> GSAGTSTATNAGPLLQRVGGLDVVKKVVELFYRKLYADPQLIKYLHDQDPMHLRAKQSMFVS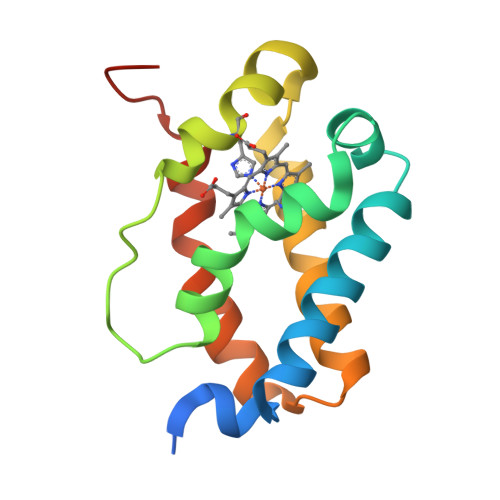WLFGPPNVPYTGKSVRIAHLRIIKQRGFSPEDFDLGMKYFEEAMTELGAPEVLRGEVMRRMLPYKDAIFTPAAGDAAEEA>[2x]ETIASELKAIGKELEDQKKEENIQIAKIAKEKFDFLSTFKVGPYDLIDEDIQMKIKRTLYSSLDYKKENIEKLKEILEIL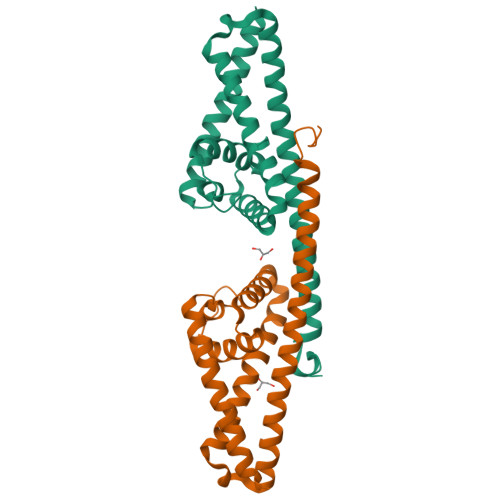KKNSEHYNIIGRLIYHISWGIQFQIEQNLELIQNGVENLSQEESKSLLMQIKSNLEIKQRLKKTLNETLKVYNQNTQDNEKILAEHFNKYYKDFDTLKPAF> MNDIYARRLAQTSMFHQLMRSHGTLWAATQVTK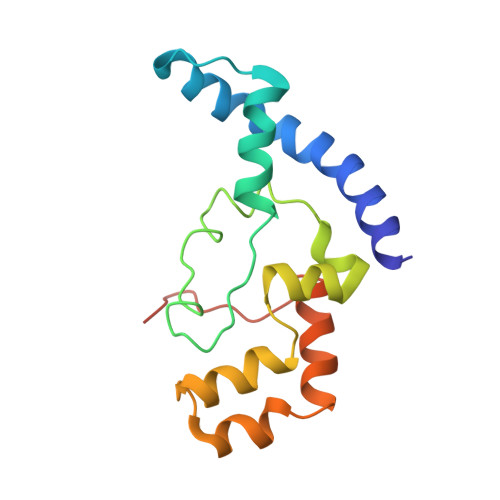EKLNLAFVKEEMMRVNGRRAMPLLIGAAANENLNDTHFTHLTEHCAWTESARAFAVQRQTPLTQHIASMGRMAETITQAKTASTSQLLFNEHLARIDGISEFEEEPFVDDEDDS>GSHMGRFADFFRIETEIQRLDNPAGILANGKKCDFTGACDPVVTAFLDLESPLSPWPGSVAASKWKTIFEATDQNSPTIGRSVIRDMCGGSASNVNLRVLVNDADSLSSQDEIGKFSCLFQLDARDVAMDSLSAQW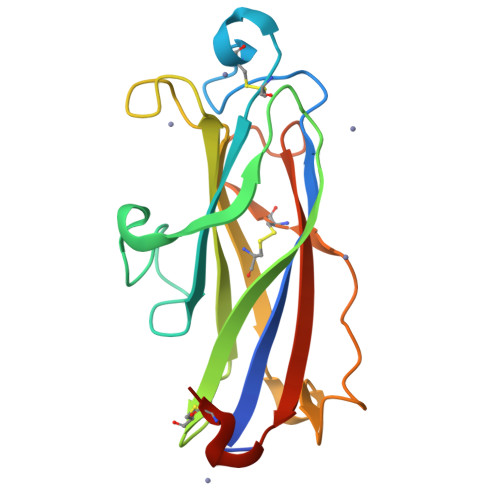GPSTECTAEAQQGKIRLFARRRAFEIPSTSCRAPSSL[2x]>MMLSLRPYEFWFVTGSQHLYGEEALKQVEEHSRIMVNEWNRDSVFPFPFVFKSVVTTPEEIRRVCLEANASEQCAGVVTWMHTFSPAKMWIGGLLELRKPLLHLHTQFNRDIPWDSIDMDFMNLNQSAHGDREYGFIGARMGVARKVVVGHWEDPEVRERLAKWMRTAVAFAESRNLKVARFGDNMREVAVTEGDKVGAQIQFGWSVNGYGIGDLVQYIRDVSEQKVNELLDEYEELYDIVPAGRQEGPVRESIREQARIELGLKAFLQDGNFTAFTTTFEDLHGMKQLPGLAVQ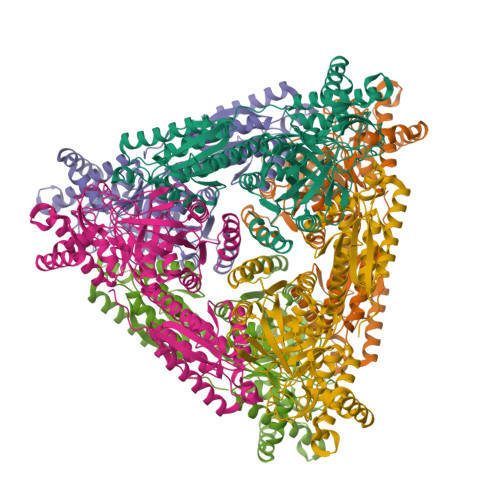RLMAEGYGFGGEGDWKTAALVRLMKVMADGKGTSFMEDYTYHFEPGNELILGAHMLEVCPTIAATRPRVEVHPLSIGGKEDPARLVFDGGEGAAVNASLIDLGHRFRLIVNEVDAVKPEHDMPKLPVARILWKPRPSLRDSAEAWILAGGAHHTCFSFAVTTEQLQDFAEMAGIECVVINEHTSVSSFKNELKWNEVFWRGR[6x]>[2x]MDHLPIFCQLRDRDCLIVGGGDVAERKARLLLEAGARLTVNALTFIPQFTVWANEGMLTLVEGPFDETLLDSCWLAIAATDDDTVNQRVSDAAESRRIFCNVVDAPKAASFIMPSIIDRSPLMVAVSAGGTSPVLARLLREKLESLLPQHLGQVARYAGQLRARVKKQFATMGERRRFWEKFFVNDRLAQSLANADEKAVNATTERLFSEPLDHRGEVVLVGAGPGDAGLLTLKGLQQIQQADIVVYDRLVSDDIMNLVRRDADRVFVGKRAGYHCVPQEEINQILLREAQKGKRVVRLKGGDPFIFGRGGEELETLCHAGIPFSVVPGITAASGCSAYSGIPLTHRDYAQSVRLVTGHLKTGGELDWENLAAEKQTLVFYMGLNQAATIQEKLIAFGMQADMPVALVENGTSVKQRVVHGVLTQLGELAQQVESPALIIVGRVVALRDKLNWFSNH

Siroheme is the modified isobacteriochlorin tetrapyrrole used by siroheme-dependent sulfite and nitrite reductases (SiR/NiRs) in catalyzing the six-electron reduction of sulfite to sulfide or nitrite to ammonia. CysG is encoded by a gene fusion between a C-terminal SUMT (CysGA) and an N-terminal bifunctional dehydrogenase/ferrochelatase (CysGB). The N-terminal enzyme module, CysGB, is a three-domain bifunctional dehydrogenase/ATP-independent class III ferrochelatase12 that performs the final two steps of siroheme biosynthesis. The C-terminal enzyme module, CysGA, is homologous to a well-studied class of SAM-dependent uro’gen III methyltransferases (SUMTs) that catalyzes the methylations to generate precorrin-210,13.

We attempted to trap the co-sirohydrochlorin product by co-soaking sirohydrochlorin and cobalt. The resulting structure was lower resolution than the other structures and the closed active site that bound precorrin-2 and sirohydrochlorin showed no additional density. The open active site, however, contained a large, flat density that we interpreted as corresponding to a loosely bound product, sitting nearly perpendicularly to the position of the intermediates in the closed active site. Co-sirohydrochlorin was not bound deeply in the open cavity so its density was more diffuse than that for the other tetrapyrroles, but sufficient to assign the central plane of the tetrapyrrole as nearly orthogonal to precorrin-2 and sirohydrochlorin. Then, once metal is inserted, there would be steric overlap between the metal and P133, leading to product release, as captured in the weakly bound co-sirohydrochlorin. Given the differences between the binding poses of the unmetallated precorrin-2/sirohydrochlorin and the metallated tetrapyrrole, we propose a mechanism for product release: steric clash between the metal and the P133 platform induce the tetrapyrrole to break its extensive interactions with the binding pocket, allowing movement of helix 6 so the product can diffuse out of the active site.>MTSAEMTSPNNNSEHQAIAKMRTMIEGFDDISHGGLPIGRSTLVSGTSGTGKTLFSIQFLYNGIIEFDEPGVFVTFEETPQDIIKNARSFGWDLAKLVDEGKLFILDASPDPEGQEVVGGFDLSALIERINYAIQKYRARRVSIDSVTSVFQQYDASSVVRRELFRLVARLKQIGATTVMTTERIEEYGPIARYGVEEFVSDNVVILRNVLEGERRRRTLEILKLRGTSHMKGEYPFTITDHGINIFPLGAMRLTQRSSNVRVSSGVVRLDEMCGGGFFKDSIILATGATGTGKTLLVSRFVENACANKERAILFAYEESRAQLLRNAYSWGMDFEEMERQNLLKIVCAYPESAGLEDHLQIIKSEINDFK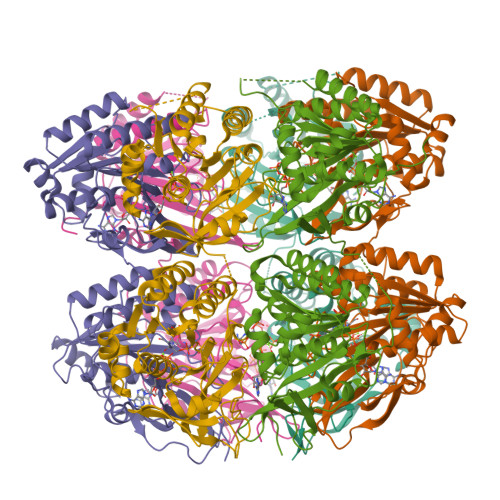PARIAIDSLSALARGVSNNAFRQFVIGVTGYAKQEEITGLFTNTSDQFMGAHSITDSHISTITDTIILLQYVEIRGEMSRAINVFKMRGSWHDKAIREFMISDKGPDIKDSFRNFERIISGSPTRITVDEKSELSRIVRGVQEKGPES[6x]[({[4-(1H-tetrazol-5-yl)phenyl]sulfonyl}amino)methyl]boronic acid | C8 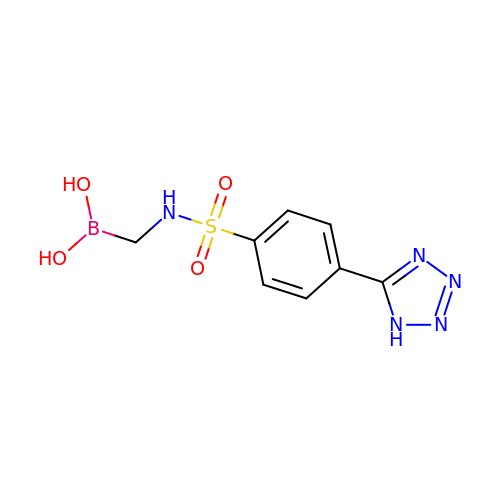H10 B N5 O4 S | SHNAIZGISNDQJQ-UHFFFAOYSA-N> GQRWELALGRFWDYLRWVQTLSEQVQEELLSSQVTQELRALMDETMKELKAYKSELEEQLTPVAEETRARLSKELQAAQARLGADMEDVRGRLVQYR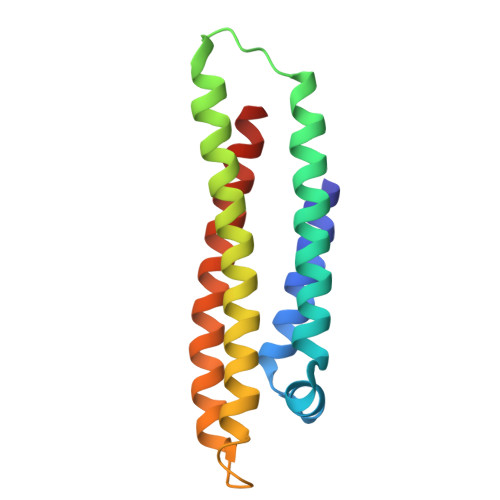GEVQAMLGQSTEELRVRLASHLRKLRKRLLRDADDLQKRLAVYQAGA>[2x]GSHMGQDIQLIPPLINLLMSIEPDVIYAGHDNTKPDTSSSLLTSLNQLGERQLLSVVKWSKSLPGFRNLHIDDQITLIQYSWMSLMVFGLGWRSYKHVSGQMLYF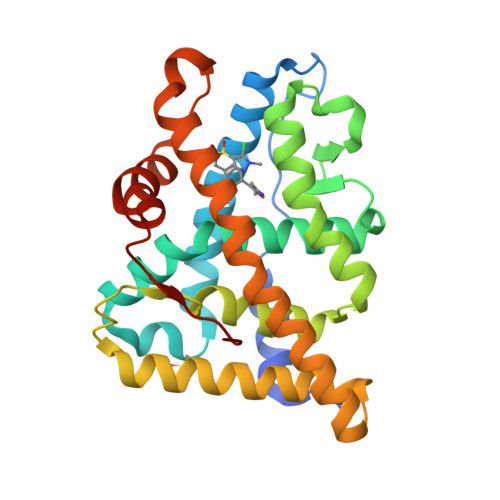APDLILNEQRMKESSFYSLCLTMWQIPQEFVKLQVSQEEFLCMKVLLLLNTIPLEGLRSQTQFEEMRSSYIRELIKAIGLRQKGVVSSSQRFYQLTKLLDNLHDLVKQLHLYCLNTFIQSRALSVEFPEMMSEVIAAQLPKILAGMVKPLLFHKK>AFKRHIDRLPIIPADAKKHNVTCHFCIVGCGYHAYTWPINKQGGTDPQNNIFGVDLSEQQQAESDAWYSPSMYNVVKQDGRDVHVVIKPDHECVVNSGLGSVRGARMAETSFSEARNTQQQRLTDPLVWRYGQMQPTSWDDALDLVARVTAKIVKEKGEDALIVSAFDHGGAGGGYENTWGTGKLYFEAMKVKNIRIHNRPAYNSEVHGTRDMGVGELNNCYEDAELADTIVAVGTNALETQTNYFLNHWIPNLRGESLGKKKELMPEEPHEAGRIIIVDPRRTVTVNACEQTAGADNVLHLAINSGTDLALFNALFTYIADKGWVDRDFIDKSTLREGTARPPLYPARGVSEANPGHLSSFEDAVEGCRMSIEEAAEITGLDAAQIIKAAEWIGMPKEGGKRRRVMFGYEKGLIWGNDNYRTNGALVNLALATGNIGRPGGGVVRLGGHQEGYVRPSDAHVGRPAAYVDQLLIGGQGGVHHIWGCDHYKTTLNAHEFKRVYKKRTDMVKDAMSAAPYGDREAMVNAIVDAINQGGLFAVNVDIIPTKIGEACHVILPAATSGEMNLTSMNGERRMRLTERYMDPP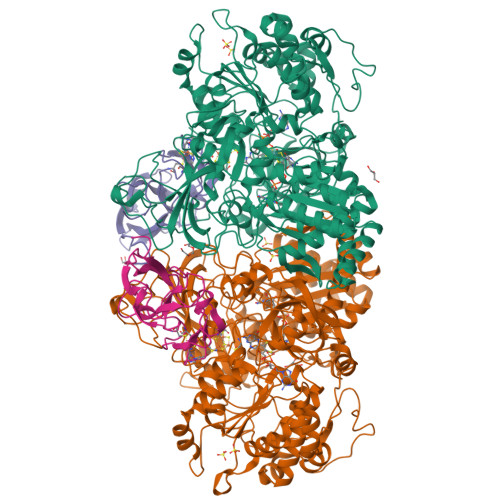GQSMPDCLIAARLANTMERVLTEMGDVGYAAQFKGFDWQTEEDAFMDGYNKNAHGGEFVTYERLSAMGTNGFQEPATGFTDGKIEGTQRLYTDGVFSTDDGKARFMDAPWRGLQAPGKQQQKDSHKYLINNGRANVVWQSAYLDQENDFVMDRFPYPFIEMNPEDMAEAGLKEGDLVEIYNDAGATQAMAYPTPTARRGETFMLFGFPTGVQGNVTSAGTNELIIPNYKQTWGNIRKISDAPRNVAHLSFKSKEYQS[4x];>AAGVEYPANRLANISELTLNEPLDVAYPDEDAAGVLLKLGTRVEGGVGPDGDIVGFSTICPHKGAPLSYSADNKTFNCPGHFSVFDPEKGGQQVWGQATQNLPQYVLRVADNGDIFAEGVDELIYGRLSNVL[4x]>GPNCAPGQKVKLFRASEPILSVLMWGVNHTINELSNVPVPVMLMPDDFKAYSKIKVDNHLFNKENLPSRFKFKEYCPMVFRNLRERFGIDDQDYQNSVTRSAPINSDSQGRCGTRFLTTYDRR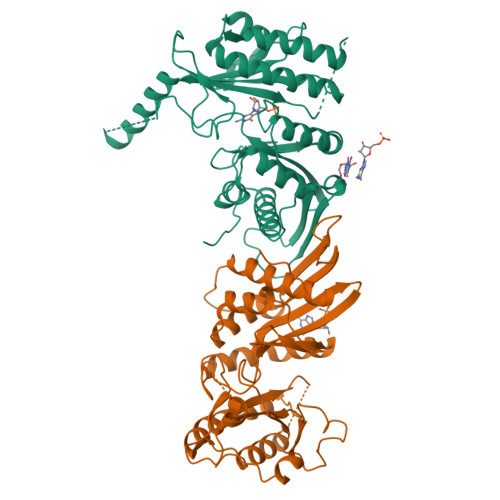FVIKTVSSEDVAEMHNILKKYHQFIVECHGNTLLPQFLGMYRLTVDGVETYMVVTRNVFSHRLTVHRKYDLKGSTVAREASDKEKAKDLPTFKDNDFLNEGQKLHVGEESKKNFLEKLKRDVEFLAQLKIMDYSLLVGIHDVDRAEQEEMEVEERAEDEECENDGVGGNLLCSYGTPPDSPGNLLSFPRFFGPGEFDPSVDVYAMKSHESSPKKEVYFMAIADILTPYDTKKKAAHAAKTVKHGAGAEISTVNPEQYSKRFNEFMSNILT[2x]> SVTVKRIIDNTVIVPKLPANEDPVEYPADYFRKSKEIPLYINTTKSLSDLRGYVYQGLKSGNVSIIHVNSYLYGALKDIRGKLDKDWSSFGINIGKAGDTIGIFDLVSLKALDGVLPDGVSDASRTSADDKWLPLYLLGLYRVGRTQMPEYRKKLMDGLTNQCKMINEQFEPLVPEGRDIFDVWGNDSNYTKIVAAVDMFFHMFKKHECASFRYGTIVSRFKDCAALATFGHLCKITGMSTEDVTTWILNREVADEMVQMMLPGQEIDKADSYMPYLIDFGLSSKSPYWSVKNPAFHFWGQLTALLLRSTRARNARQPDDIEYTSLTT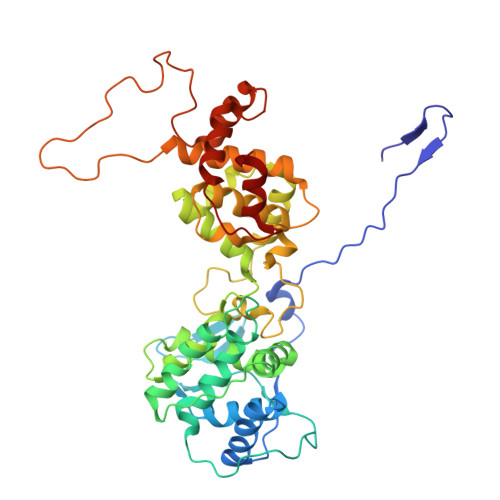AGLLYAYAVGSSADLAQQFCVGDNKYTPDDSTGGLTTNAPPQGRDVVEWLGWFEDQNRKPTPDMMQYAKRAVMSLQGLREKTIGKYAKSEFDK>MGSSHHHHHHSQDPNSMLSVGATTTATRLTGWGRTAPSVANVLRTPDAEMIVKAVARVAESGGGRGAIARGLGRSYGDNAQNGGGLVIDMTPLNTIHSIDADTKLVDIDAGVNLDQLMKAALPFGLWVPVLPGTRQVTVGGAIACDIHGKNHHSAGSFGNHVRSMDLLTADGEIRHLTPTGEDAELFWATVGGNGLTGIIMRATIEMTPTSTAYFIADGDVTASLDETIALHSDGSEARYTYSSAWFDAISAPPKLGRAAVSRGRLATVEQLPAKLRSEPLKFDAPQLLTLPDVFPNGLANKYTFGPIGELWYRKSGTYRGKVQNLTQFYHPLDMFGEWNRAYGPAGFLQYQFVIPTEAVDEFKKIIGVIQASGHYSF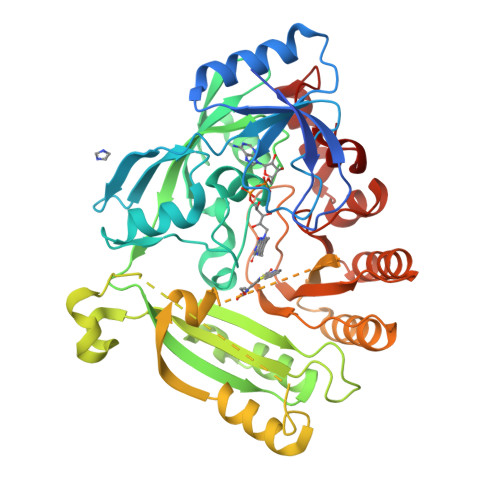LNVFKLFGPRNQAPLSFPIPGWNICVDFPIKDGLGKFVSELDRRVLEFGGRLYTAKDSRTTAETFHAMYPRVDEWISVRRKVDPLRVFASDMARRLELL[2x]5-Se-methyl-5-seleno-beta-D-ribofuranose | C6 H12 O4 Se | 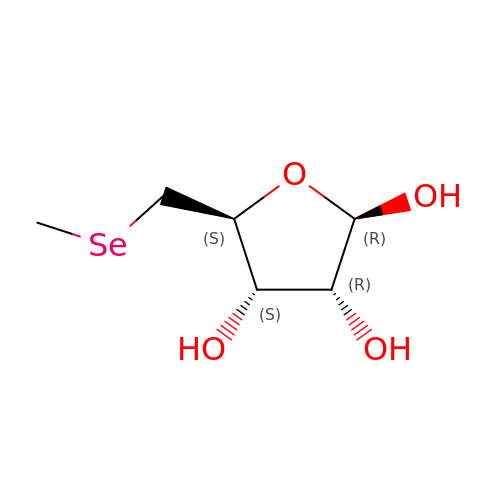UFNQFLPLDXICBS-KVTDHHQDSA-N The key enzyme in the salvage pathway is hypoxanthine–guanine–(xanthine) phosphoribosyltransferase (HG(X)PRT)4. Inhibition of hypoxanthine–guanine–xanthine phosphoribosyltransferase activity decreases the pool of 6-oxo and 6-amino purine nucleoside monophosphates required for DNA and RNA synthesis, resulting in a reduction in cell growth. Five compounds synthesized here that contain a purine base covalently linked by a prolinol group to one or two phosphonate groups have Ki values ranging from 3 nM to >10 μM, depending on the structure of the inhibitor and the biological origin of the enzyme. X-ray crystal structures show that, on binding, these prolinol-containing inhibitors stimulated the movement of active site loops in the enzyme.

5 is a nanomolar inhibitor of both human HGPRT and TBrHGPRT1 (Ki = 3 nM). In human HGPRT, it is the phosphonate group attached to the carbon atom of the prolinol ring that enters the 5′-phosphate binding pocket whereas, when 5 is bound to TBrHGPRT1, it is the group that is attached to the nitrogen atom. Perhaps, these interactions are not possible in the structure of TBrHGPRT1 and, hence, the change in orientation of the inhibitor. It is hypothesized that the loop surrounding this 5′-phosphate binding site is less flexible in TBr than the counterpart in the human enzyme. Therefore, this loop is unable to move out to accommodate the longer linker and, as a result, the two phosphonate groups occupy alternate binding pockets in the human and Tbr enzymes. The carbonyl group in the TBrHGPRT1·5 complex does not form any interactions with active site residues. There are no magnesium ions in the TBrHGPRT1·5 complex, and, as such, divalent metal ions do not play any role in anchoring this molecule in the active site. In the case of the TBr enzyme, the phosphonate group is held in position by only three hydrogen bonds. However, these bonds, together with the other interactions in the active site, are sufficient to result in a high affinity of the compound for the enzyme. The prolinol ring in TbrHGPRT1 is rotated by ∼90° compared to its binding to the human counterpart. The TBrHGPRT1·4 complex refines as a dimer, while the TBrHGPRT1·5 complex refines as two dimers.

>ACKYDFATSVLFTEAELHTRMRGVAQRIADDYSNCNLKPLENPLVIVSVLKGSFVFTADMVRILGDFGVPTRVEFLRASSYGHDTKSCGRVDVKADGLCDIRGKHVLVLEDILDTALTLREVVDSLKKSEPASIKTLVAIDKPGGRKIPFTAEYVVADVPNVFVVGYGLDYDQSYREVRDVVILKPSVYETWGKELERRKA[4x]>GPHMTRLGLEFFDQPAVPLARAFLGQVLVRRLPNGTELRGRIVETEAYLGPEDEAAHSRGGRQTPRNRGMFMKPGTLYVYIIYGMYFCMNISSQGDGACVLLRALEPLEGLETMRQLRSTLRKGTASRVLKDRELCSGPSKLCQALAINKSFDQRDLAQDEAVWLERGPLEPSEPAVVAAARVGVGHAGEWAR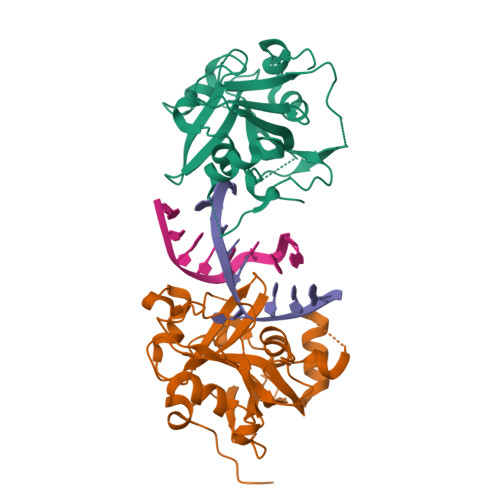KPLRFYVRGSPWVSVVDRVAEQDTQA[2x]>MAHHHHHHMVNVAVIGAAGGIGQSLSLLLLRELPFGSTLSLYDVVGAPGVAADLSHIDRAGITVKHAAGKLPPVPRDPALTELAEGVDVFVIVAGVPRKPGMTRDDLFNVNAGIVMDLVLTCASVSPNACFCIVTNPVNSTTPIAAQTLRKIGVYNKNKLLGVSLLDGLRATRFINNARHPLVVPYVPVVGGHSDVTIVPLYSQIPGPLPDESTLKEIRKRVQVAGTEVVKAKAGRGSATLSMAEAGARFTMHVVKALMGLDTPMVYAYVDTDGEHECPFLAMPVVLGKNGIERRLPIGPITTVEKEMLEEAVGVVKKNIAKGETFARSKL[4x]

Having no protein synthetic abilities, peroxisomes import all required enzymes from the cytosol through a peroxin (Pex) import system. Peroxisome targeting sequence 1 (PTS1)-tagged cargo is recognized by cytosolic receptor, Pex5. The cargo-Pex5 complex docks at the peroxisomal membrane translocon, composed of Pex14 and Pex13, facilitating translocation into the peroxisomal lumen. MDH is a crucial enzyme for the glycolysis auxiliary pathway, maintaining the pool of malate/oxaloacetate.

The resulting maps facilitated de novo model building for MDH, forming a tetramer of ~10 nm diameter. The tetramer is composed of two dimers related by dihedral (D2) symmetry. The peroxisomal targeting signal 1 (PTS1) motifs of all MDH subunits are found at the periphery of the tetramer and are equally accessible to the solvent. The additional density is observed only at sites occupied by Pex5, and not at the vacant PTS1 sites, indicating that it corresponds to a fragment of the Pex5457-489 loop. Additionally, the density was absent in the map of MDH tetramer solved in this study, further suggesting it originates from Pex5.> MSELYQAKSETRSTITSSLKGIQPYKPTKATIWSRADALKVNEYDPTTTQPLVSGDFPVMSDEVFIWDTMPLRDIDGNIASVNGWSVIFTLTADRNPTAPEYQDEQGNYDITLDWNDRHGRAKMYFWYSRTGKDWIIGGRVMAEGVSPTAREWAGTPVLLNERGEIDLYYTAVTPGATVVKVRGRVVTTENGVEMVGFKKVKSLFEADGKMYQTESQNPYWAFRDPCPFRDPKSGKLYMLFEGNVAGERGSHVVGPDELGDVPPGYEDAGNSHFQTGCIGIAVCRDEDGDDWELLPPLITAVGVNDQTERPHFVFQDGKYYLF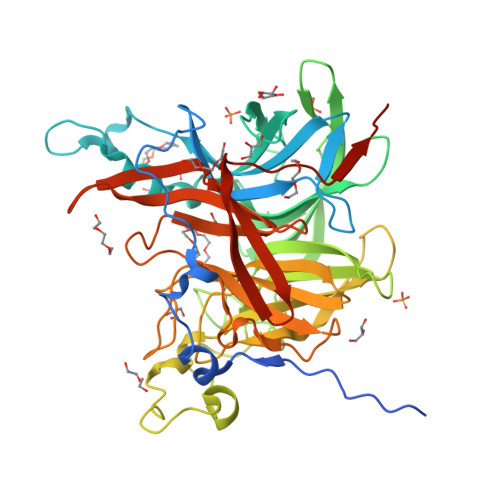TISHKFTYGDGLTGPDGVYGFVSENLFGPYVPLNGSGLVLGNPPSQPYQTYSHYVMPNGLVTSFIDSVPTGEDSYRIGGTEAPTVLIKLKGAQTFVLEEFDYGYIPPMIDVKVEHHHHHH> MVVSLAGRDLLCLQDYTAEEIWTILETAKMFKIWQKIGKPHRLLEGKTLAMIFQKPSTRTRVSFEVAMAHLGGHALYLNAQDLQLRRGETIADTARVLSRYVDAIMARVYDHKDVEDLAKYATVPVINGLSDFSHPCQALADYMTIWEKKGTIKGVKVVYVGDGNNVAHSLMIAGTKLGADVVVATPEGYEPDEKVIKWAEQNAAESGGSFELLHDPVKA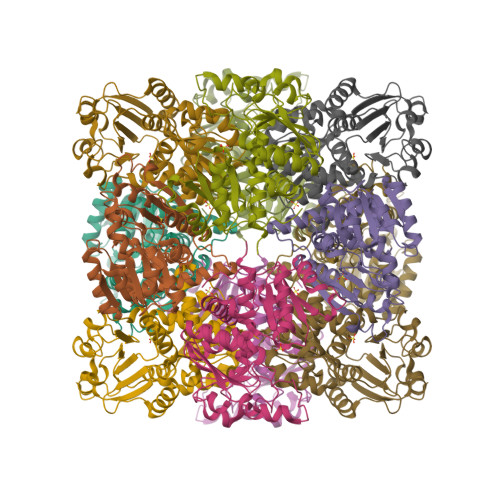VKDADVIYTDVWASMGQEAEAEERRKIFRPFQVNKDLVKHAKPDYMFMHCLPAHRGEEVTDDVIDSPNSVVWDQAENRLHAQKAVLALVMGGIKF The larger, 169-residue LspA is a key enzyme in the lipoprotein processing pathway of Pseudomonas aeruginosa. LspA functions to release the signal peptide from prolipoproteins and is inhibited by the natural macrocyclic antibiotics, globomycin, and myxovirescin. It is a promising target for the development of drugs that combat antimicrobial resistance. In meso crystal structures of LspA in complex with globomycin and myxovirescin reveal that the enzyme consists of four transmembrane helices with periplasmic extensions that include an amphiphilic β sheet region, referred to as the β cradle, and a flexible loop with a short periplasmic helix.

In meso crystallization trials with the doubly labeled enzyme produced crystals and an X-ray diffraction structure to 3 Å resolution with a minimum of optimization. As expected, the structures of the labeled and unlabeled protein are virtually identical with a root-mean-square deviation of 0.36 Å for backbone Cα atoms. Furthermore, LspA peptidase activity was unaffected, and the enzyme was inhibited by globomycin as judged by the FRET progress curves. This supports the view that the 13C/15N-labeled LspA preparation used in the ssNMR experiments was properly folded and enzymatically active. The complex used in this study was prepared by incubating detergent-solubilized 13C/15N-labeled LspA with a 10-fold molar excess of globomycin for 30 min on ice. Reconstitution of the complex into the cubic mesophase was carried out by the traditional twin-syringe mixing method. LspA solution NMR data corroborate the view that LspA undergoes considerable structural and dynamical rearrangements upon complexation with globomycin and the macrocyclic antibiotic, myxovirescin. These structural changes likely involve stabilization of the LspA backbone in a more rigid conformation.

>[4x]MPDVDRFGRLPWLWITVLVFVLDQVSKAFFQAELSMYQQIVVIPDLFSWTLAYNTGAAFSFLADSSGWQRWLFALIAIVVSASLVVWLKRLKKGETWLAIALALVLGGALGNLYDRMVLGHVVDFILVHWQNRWYFPAFNLADSAITVGAVMLALDMFRSKKSGEAAHG;>[4x]LISTX> SALRETVVEVPQVTWEDIGGLEDVKRELQELVQYPVEHPDKFLKFGMTPSKG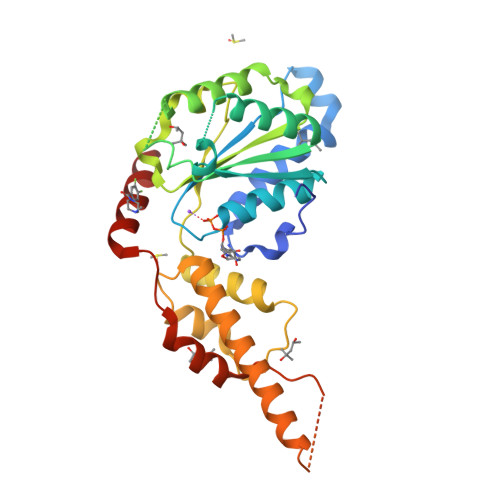VLFYGPPGCGKTLLAKAIANECQANFISIKGPELLTMWFGESEANVREIFDKARQAAPCVLFFDELDSIAKARGGNIGDGGGAADRVINQILTEMDGMSTKKNVFIIGATNRPDIIDPAILRPGRLDQLIYIPLPDEKSRVAILKANLRKSPVAKDVDLEFLAKMTNGFSGADLTEICQRACKLAIRESIESEIRRERERQTNPSAMEVEEDDPVPEIRRDHFEEAMRFARRSVSDNDIRKYEMFAQTLQQ> SMIFKPEELRQALMPTLEAL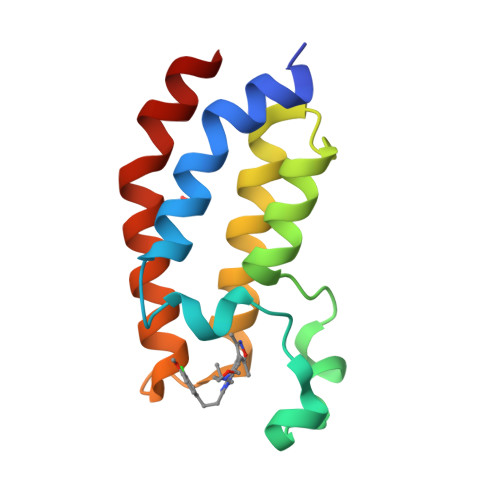YRQDPESLPFRQPVDPQLLGIPDYFDIVKSPMDLSTIKRKLDTGQYQEPWQYVDDIWLMFNNAWLYNRKTSRVYKYCSKLSEVFEQEIDPVMQSLG4-(4-methyl-2-methylsulfanyl-1~{H}-imidazol-5-yl)-~{N}-(4-morpholin-4-ylphenyl)pyridin-2-amine 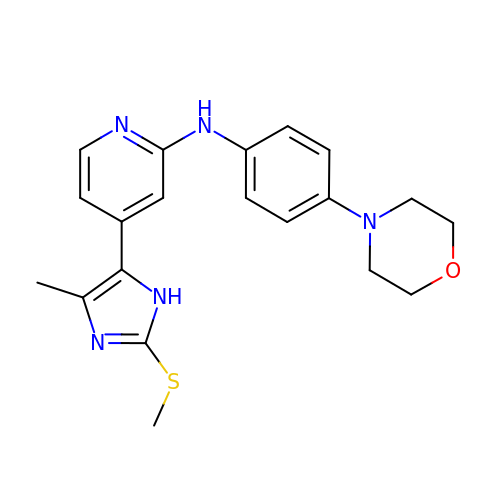| C20 H23 N5 O S | IATSSYNKRCFJAY-UHFFFAOYSA-N> LLVVGPKFIRANQEYTLVISNFNSQLSKVDLLLKLEGETDNGLSVLNVTKMVDVRRNMNRMINFNMPEDLTAGNYKITIDGQRGFSFHKEAELVYLSKSISGLIQVDKPVFKPGDTVNFRVIVLDTELKPPARVKSVYVTIRDPQRNVIRKWSTAKLYAGVFESDLQIAPTPMLGVWNISVEVEGEELVSKTFEVKEYVLSTFDVQVMPSVIPLEEHQAVNLTIEANYHFGKPVQGVAKVELYLDDDKLKLKKELTVYGKGQVELRFDNFAMDADQQDVPVKVSFVEQYTNRTVVKQSQITVYRYAYRVELIKESPQFRPGLPFKCALQFTHHDGTPAKGISGKVEVSDVRFETTTTSDNDGLIKLELQPSEGTEQLSIHFNAVDGFFFYEDVNKVETVTDAYIKLELKSPIKRNKLMRFMVTCTERMTFFVYYVMSKGNIIDAGFMRPNKQPKYLLQLNATEKMIPRAKILIATVAGRTVVYDFADLDFQELRNNFDLSIDEQEIKPGRQIELSMSGRPGAYVGLAAYDKALLLFNKNHDLFWEDIGQVFDGFHAINENEFDIFHSLGLFARTLDDILFDSANEKTGRNALQSGKPIGKLVSYRTNFQESWLWKNVSIGRSGSRKLIEVVPDTTTSWYLTGFSIDPVYGLGIIKKPIQFTTVQPFYIVENLPYSIKRGEAVVLQFTLFNNLGAEYIADVTLYNVANQTEFVGRPNTDLSYTKSVSVPPKVGVPISFLIKARKLGEMAVRVKASIMLGHETDALEKVIRVMPESLVQPRMDTRFFCFDDHKNQTFPINLDINKKADSGSTKIEFRLNPNLLTTVIKNLDHLLGVPTGCGEQNMVKFVPNILVLDYLHAIGSKEQHLIDKATNLLRQGYQNQMRYRQTDGSFGLWETTNGSVFLTAFVGTSMQTAVKYISDIDAAMVEKALDWLASKQHFSGRFDKAGAEYHKEMQGGLRNGVALTSYVLMALLENDIAKAKHAEVIQKGMTYLSNQFGSINNAYDLSIATYAMMLNGHTMKEEALNKLIDMSFIDADKNERFWNTTNPIETTAYALLSFVMAEKYTDGIPVMNWLVNQRYVTGSFPSTQDTFVGLKALTKMAEKISPSRNDYTVQLKYKKSAKYFKINSEQIDVENFVDIPEDTKKLEINVGGIGFGLLEVVYQFNLNLVNFENRFQLDLEKQNTGSDYELRLKVCASYIPQLTDRRSNMALIEVTLPSGYVVDRNPISEQTKVNPIQKTEIRYGGTSVVLYYDNMGSERNCFTLTAYRRFKVALKRPAYVVVYDYYNTNLNAIKVYEVDKQNLCEICDEEDCPAECGGHHHHHH

Anopheles gambiae thioester-containing protein 1 (TEP1) is a complement-like protein that plays a central role in the opsonization of gram-negative bacteria in the hemolymph. TEP1 also binds to the surface of Plasmodium ookinetes that traverse the midgut epithelium following ingestion of an infectious blood meal, targeting those ookinetes for lysis and, in certain mosquito strains, melanization. TEP1 is composed of a series of eight macroglobulin (MG) domains, the β-sheet CUB domain and α-helical thioester domain (TED). The TED contains an intramolecular β-cysteinyl-γ-glutamyl thioester bond that is protected from inadvertent hydrolysis by sequestration within a protein-protein interface formed by the TED and MG8 domains.

The refractory allele, TEP1*R1, has been expressed in vitro and utilized in structural and functional studies. The TEP1*S1 and TEP1*R1 proteins share 93% sequence identity with the majority of amino acid differences being confined to three hypervariable loops within the TED domain. The TEP1*R1 catalytic loop contains a sequence of five residues including Lys 966 and Glu 970 (966KAGAE970). TEP1*S1 Glu 966 adopts a different conformation than Lys 966 in TEP1*R1, directed into a pocket occupied by a Cl− ion in TEP1*R1, within hydrogen bonding distance of Ser 921 Oγ and Phe 923 N (the same conformation observed for Glu 1098 in complement factor C3). In contrast Ser 921 is within hydrogen bonding distance of TEP1*R1 Tyr 971 but not TEP1*S1 Trp 971. The S1108R substitution does not cause any perturbation in the interface however, the Arg side chain adopts a conformation within hydrogen bonding distance of the carbonyl oxygen of Tyr 1307 instead of a water molecule as seen in TEP1*R1. The remaining 23 polymorphisms are generally localized in short loops between the TED α-helices and introduce no significant alteration to the structure, with the possible exception of four (F960S, E1005V, K1009V, T1012N) on the face of helix α7 and adjacent to the post-α5 turn that form a crystal contact within the TEP1*R1 structure. The half-life of TEP1*S1cut is 8.5 h, significantly shorter than the half-life of TEP1*R1cut (6.5 days), suggesting that TEP1*S1cut is more susceptible to hydrolysis of the thioester bond than TEP1*R1cut. TEP1*R1cut also forms a complex with LRIM1/APL1C that presumably contains an active thioester by a spontaneous conformational change with a half-life of 6.5 days at 20°C. Residues in the new TEP1*R1 and TEP1*S1 models are numbered according to the complete peptide chain (including signal peptide) for comparison with other reports.> LVATT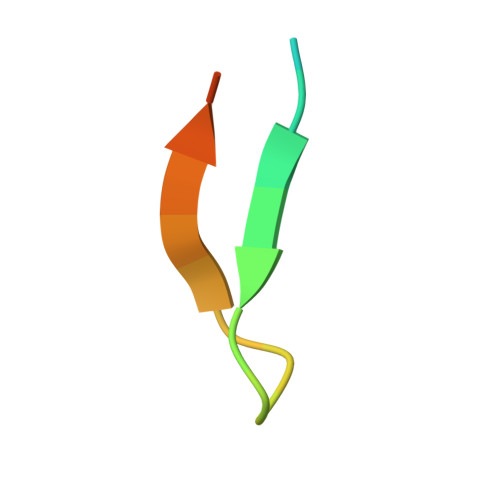SSKIYDNKNQLIADLGSER>MAPKKVLLALTSYNDVFYSDGMKTGVFVVEALHPFNTFRKEGFEVDFVSETGKFGWDEHSLAKDFLNGQDETDFKNKDSDFNKTLAKIKTPKEVNADDYQIFMASAGHGTLFDYPKAKDLQDIASEIYANGGVVAAVCHGPAMFDGLTDKKTGRPLIEGKSIT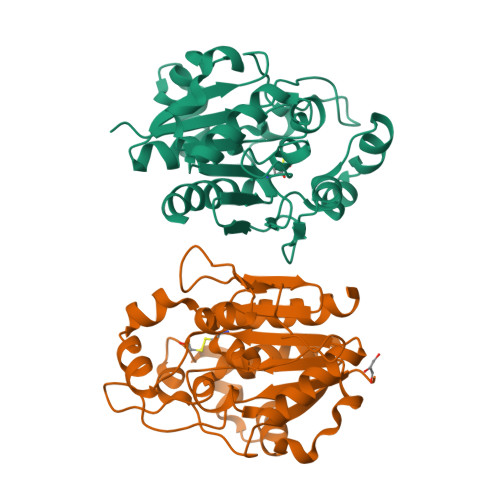GFTDVGETIMGVDSILKAKNLATVEDVAKKYGAKYLAPVGPWDDYSITDGRLVTGVNPASAHSTAVRSIDALKN[2x]>SMQRTVARDITLLECVGKGRYGEVWRGSWQGENVAVKIFSSRDEKSWFRETELYNTVMLRHENILGFIASDMTSRHSSTQLWLITHYHEMGSLYDYLQLTTLDTVSCLRIVLSIASGLAHLHIEIFGTQGKPAIAHRDLKSKNILVKKNGQCCIADLGLAVMHSQSTNQLDVGNNPRVGTKRYMAPEVLDETIQVDCFDSYKRVDIWAFGLVLWEVARRMVSNGIVEDYKPPFYDVVPNDPSFEDMRKVVCVDQQRPNIPNRWFSDPTLTSLAKLMKECWYQNP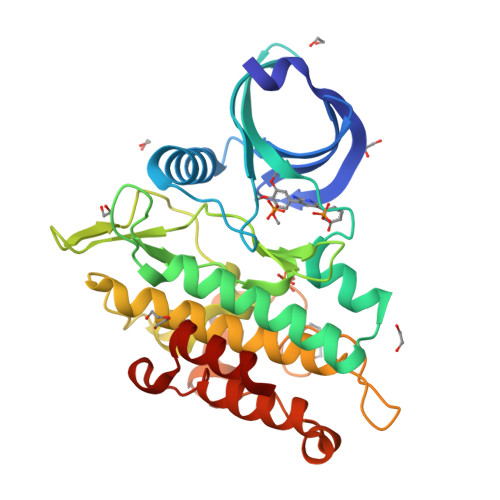SARLTALRIKKTLTKID[2x]2-[(3S)-1-oxidanyl-3H-2,1-benzoxaborol-3-yl]prop-2-enoic acid | C10 H9 B O4 | 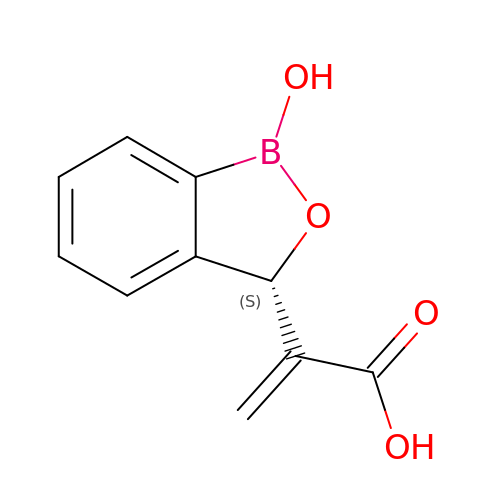BRBGRVSFRVLGNY-SECBINFHSA-N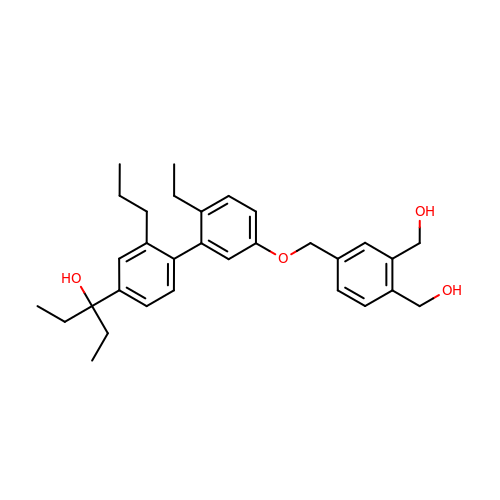3-(5'-{[3,4-bis(hydroxymethyl)benzyl]oxy}-2'-ethyl-2-propylbiphenyl-4-yl)pentan-3-ol | C31 H40 O4 | SMKNKOCYSYNJHN-UHFFFAOYSA-N>[6x]GSPEFVNSELTQLDEYGEWILEQAGEDKENLPSDVELYKKAAELDVLNDPKIGCVLAQCLFDEDIVNEIAEHNAFFTKILVTPEYEKNFMGGIERFLGLEHKDLIPLLP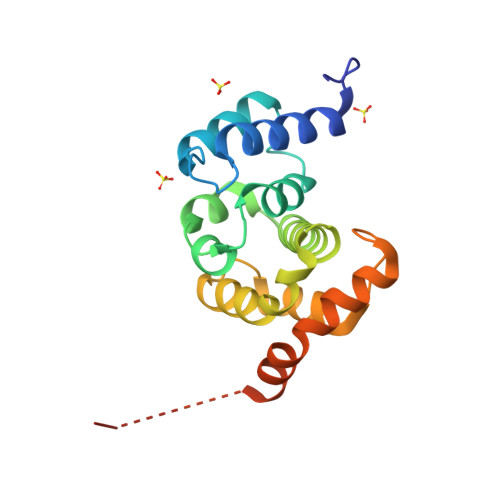KILVQLYNNDIISEEEIMRFGTKSSKKFVPKEVSKKVRRAAKPFITWLETAESDDDEEDDELERPHRD>MSQLSNQEKEYLISKALETEEGRVALAQAMANPIRVSLDYQGVGRKLLVVDPLPQGALPVYDKDVDAKAFVISKRGQVPDQVIEGDRIQVPTFEIVSYPQVRFSQVKERRFNVIDRAQQRAKADIMAVEDAEIFSLLEGAATAVNAVTISSGGLQRAALTKAFQEVEKHDLVVTKIVMNASAFADIRAWGQNEFDPVTQHEVLQTGLFGHIWTADILISKKVPQNTVYVLADPEFVGVMPIRQDIQVIPADKPEELRLGWVIYEELGLAVVNSLAIAKIS[6x];>[18x]PYVRLGYEGILNGAHDIDVAGLNGVEQLAGKFATIGANGVKLAGDNGTNAVGLFREDLGDMVNASEKASFYFRGGEYYVNISRTSLTA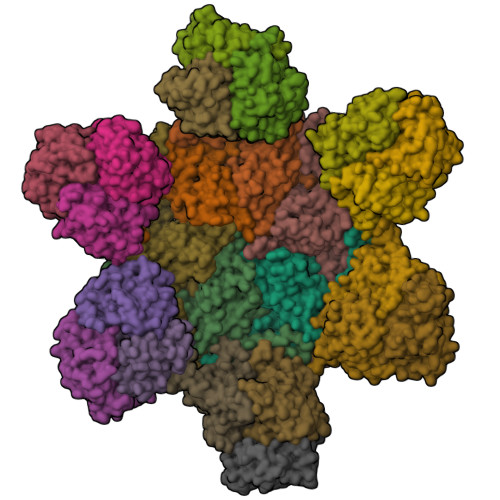AGIAAGDEITCDADGKMIKFTGTGKALGVVTHVGEYRAGNMYEKATQGVTDTDTFIGFIMYV> CTDAALAALE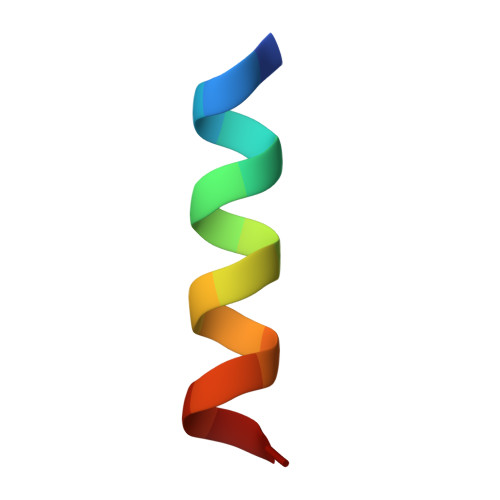YHKSNA> SLIEFGKMILEETGKLAIPSYSSYGCYCGGGGKGTPKD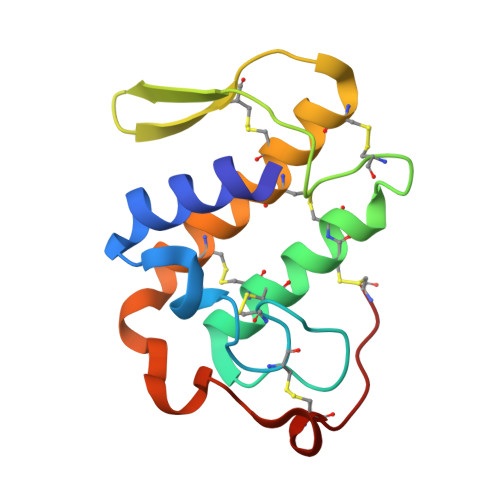ATDRCCFVHDCCYGNLPDCNPKSDRYKYKRVNGAIVCEDGTSCQNRICECDKAAAICFRQNLTTYSEKYELYPDFLCKGKIKC>[2x]GPLGSTFEEMALTTFMITKESYSKLKNSVSDVAFNRYLSLYNKYRYFSGKMDTAA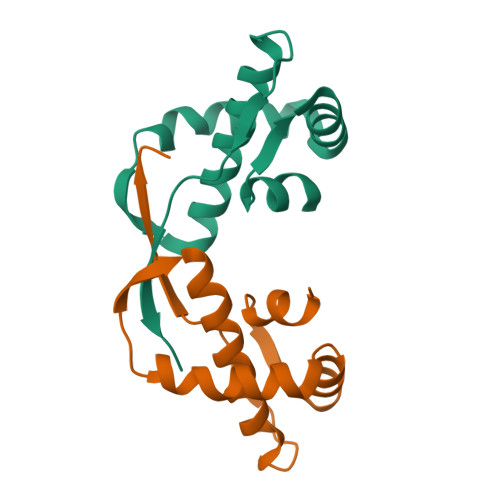YREAACSQLAKAMETFNHNNGNDVLYQPPTASVTTSFLQ(2-hydroxyethoxy)acetaldehyde 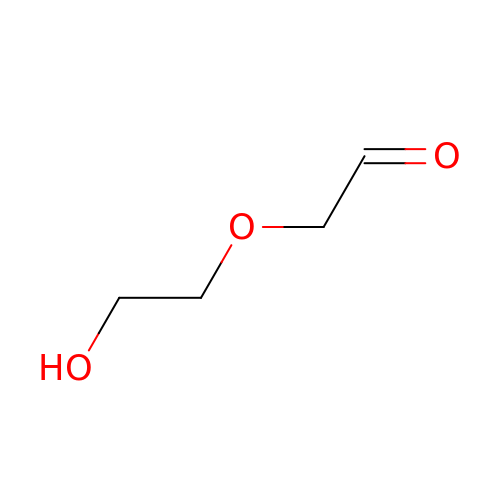| C4 H8 O3 | DSGGHBUAHUMMHN-UHFFFAOYSA-N> MKIVYWSGTGNTEKMAELIAKGIIESGKDVNTINVSDVNIDELLNEDILILGCSAMT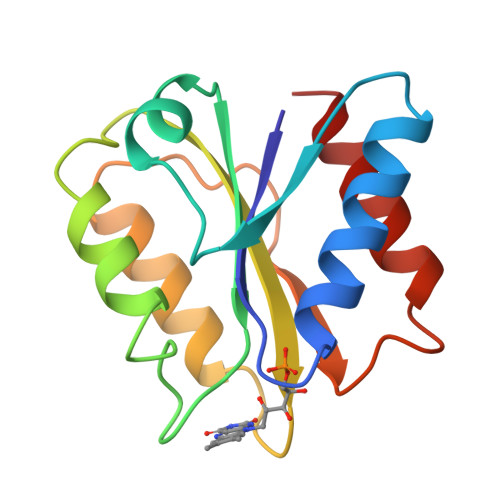DEVLEESEFEPFIEEISTKISGKKVALFGSYGWGDGKWMRDFEERMNGYGCVVVETPLIVQNEPDEAEQDCIEFGKKIANI methyl (R)-2-(1-hydroxy-1,3-dihydrobenzo[c][1,2]oxaborole-6-carboxamido)-2-phenylacetate | C17 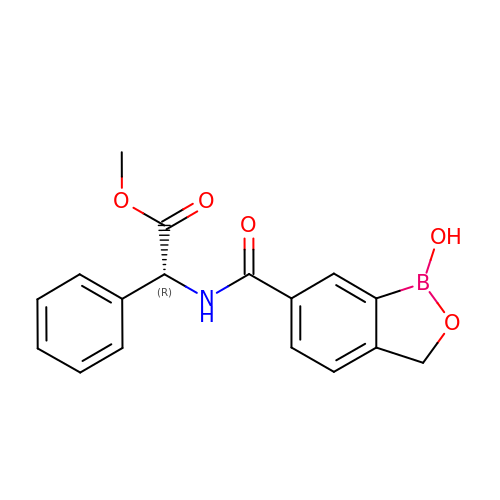H16 B N O5 | QLGLQJGWGVNAIY-OAHLLOKOSA-N NSTs belong to the SLC35 family of solute carriers and are highly conserved from simple eukaryotes like fungi and parasites to complex multicellular organisms such as plants and mammals. In the cell NSTs function to shuttle nucleotide sugars into the lumen of the ER or Golgi, in exchange for the cognate nucleoside monophosphate. GDP-mannose transport is fundamental for virulence and essential for cell survival, making the transporters attractive targets for inhibitor design.

To understand how GMP is recognised by Vrg4 we determined a co-crystal structure with GMP at 3.3 Å resolution. Vrg4 adopts a very similar pose as that for the GDP-mannose transporter (root mean square deviation ~0.47 Å between 276 Cα atoms), with the binding site open to the luminal side of the Golgi membrane and sealed shut on the cytoplasmic side through the packing together of TM6 & TM7 against TM8 and TM9. Clear mFo-DFc difference electron density was observed for the GMP ligand in three of the eight transporters in the unit cell. Unexpectedly the three GMP ligands adopt slightly different positions within the three binding sites, despite a r.m.s.d of only 0.45 Å between the three structures. In chain C, the phosphate group of the GMP molecule forms a salt bridge with a conserved lysine (K289) on TM9 and interacts with a conserved tyrosine on TM1 (Y28) through a hydrogen bond. Unlike the position of the GMP ligand in chains C and D, the molecule adopts a bent configuration, with the phosphate group now orientated towards the luminal entrance of the binding site. In this position the phosphate now interacts with a conserved serine on TM1 (S32), rather than K289, which adopts a different rotamer configuration compared to chains C and D. However, unlike the GDP-mannose ligand, GMP does not make a direct interaction to the conserved asparagines of the FYNN motif, which are ~4.5 Å away. Analysis of the apo, GMP and GDP-mannose bound structures of Vrg4 show the presence of well−ordered monoolein lipid molecules at a potential dimer interface. Our findings that GMP adopts several similar, yet discrete conformations in the binding site now provides evidence that the slower rate of transport observed for GMP vs. GDP-mannose is due to less effective coupling between the ligand and the transporter.

>[8x]MSELKTGHAGHNPWASVANSGPISILSYCGSSILMTVTNKFVVNLKDFNMNFVMLFVQSLVCTITLIILRILGYAKFRSLNKTDAKNWFPISFLLVLMIYTSSKALQYLAVPIYTIFKNLTIILIAYGEVLFFGGSVTSMELSSFLLMVLSSVVATWGDQQAVAAKAASLAEGAAGAVASFNPGYFWMFTNCITSALFVLIMRKRIKLTNFKDFDTMFYNNVLALPILLLFSFCVEDWSSVNLTNNFSNDSLTAMIISGVASVGISYCSGWCVRVTSSTTYSMVGALNKLPIALSGLIFFDAPRNFLSILSIFIGFLSGIIYAVAKQKKQQAQPLRK> MDPTPVSVSGGTIHFEGKLVNAACAVSTKSADQTVTLGQYRTASFTAIGDTTAQVPFSIVLNDCDPKVAATAAVAFSGQADNTNTNLLAVSSADNSTTATGVGIEILDNTSSPLKPDGATFSAKQALVEGTNTLRFTARYKATAAATTPGQANADATFIMKYE;> MADPTPVSVSGGTIHFEGKLVNAACAVSTKSADQTVTLGQYRTASFTAIGDTTAQV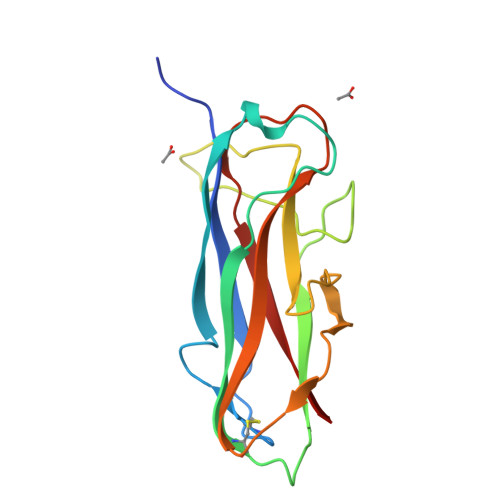PFSIVLNDCDPKVAATAAVAFSGQADNTNTNLLAVSSADNSTTATGVGIEILDNTSSPLKPDGATFSAKQALVEGTNTLRFTARYKATAAATTPGQANADATFIMKYE> SNAMSQSLRIVFAGTPDFAARHLAALLSSEHEIIAVYTQPERPAGRGKKLTASPVKTLALEHNVPVYQPENFKSDESKQQLAALNADLMVVVAYGLLLPKVVLDTPKLGCINVHGSILPRWRGAAPIQRSIWAGDSETGVTIMQMDVGLDTGDMLKIATLPIEASDTSASMYDKLAELGPQALLECLQDIAQGTAVAVKQDDGLANYAHKLSKEEARINWSDAATHIERCIRAFNPWPMSHFEVAENSIKVWQARVETRAVTQTPGT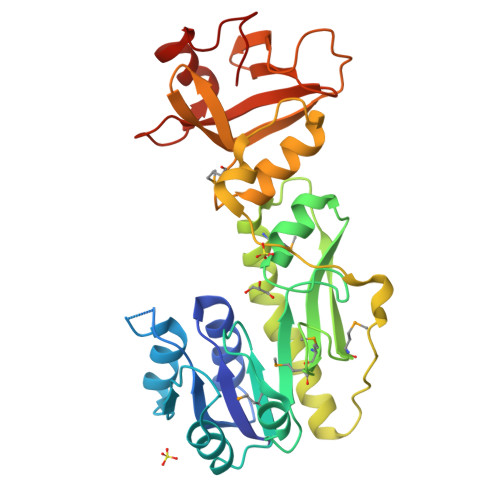IIQADKSGIYVATGQDVLVLESLQIPGKKALPVQDILNARADWFSVGSQLS>GPGSSKPFTLPILTLGELTNSRFPLPIDVLYTNPNESAIVQCQNGRCTLDGELQGTTQLLPTGICAFRGKVTQQVQDEHRGTHWNMTVTNLNG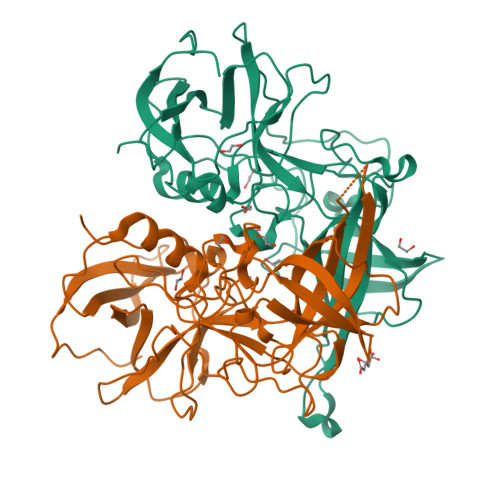TPFDPTEDVPAPLGTPDFSGQIYGVISQRNTNTVPGEGNLPANRAHEAVIATYSPKFTPKLGNIQFSTWETQDVSSGQPTKFTPVGLASVDANSHFDQWTLPSYSGALTLNMNLAPSVAPVFPGECLLFFRSFIPLKGGYGNPAIDCLMPQEWVQHLYQESAPSLSDVALVRYVNPETGRTLFEAKLHRNGFLTVARNSAGPVVAPTNGYFRFDSWVNQFYTLAPM[2x]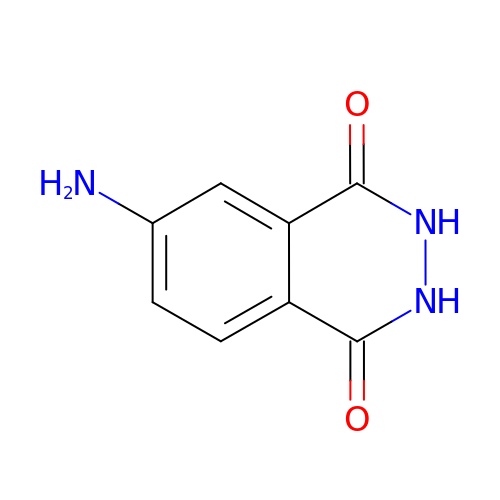4-AMINOPHTHALHYDRAZIDE | C8 H7 N3 O2 | HUDPLKWXRLNSPC-UHFFFAOYSA-N> 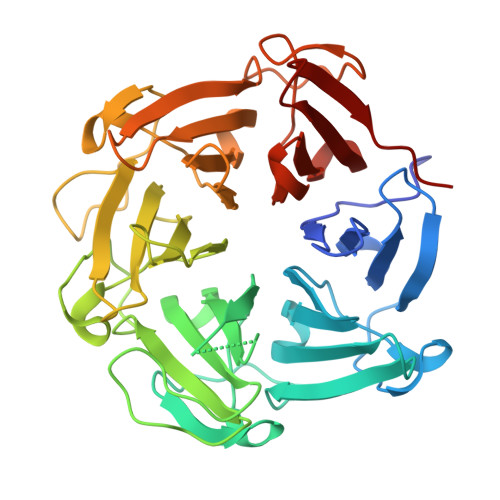MHHHHHHMSPLLFPGKVTVDQVTDRLVIADTGHHRILVVWKNGQIQYSIGGPNPGRKDGIFSESTFNSPQGVAIMNNIIYVADTENHLIRKIDLEAEKVSTVAGIGIQGTDKEGGAKGEQQPISSPWDVVFGTSGSEVQRGDILWIAMAGTHQIWALLLDSGKLPKKNELTKGTCLRFAGSGNEENRNNAYPHKAGFAQPSGLSLASEDPWSCLFVADSESSTVRTVSLKDGAVKHLVGGERDPMNLFAFGDVDGVGINAKLQHPLGVTWDKKRNLLYVADSYNHKIKVVDPKTKNCTTLAGTGDTNNVTSSSFTESTFNEPGGLCIGENGELLYVADTNNHQIKVMDLETKMVSVLPIF>[2x]MHHHHHHAAGIPMNNPAIKRIGNHITKSPEDKREYRGLELANGIKVLLISDPTTDKSSAALDVHIGSLSDPPNIAGLSHFLQHMLFLGTKKYPKENEYSQFLSEHAGSSNAFTSGEHTNYYFDVSHEHLEGALDRFAQFFLSPLFDESAKDREVNAVDSEHEKNVMNDAWRLFQLEKATGNPKHPFSKFGTGNKYTLETRPNQEGIDVRQELLKFHSAYYSSNLMAVVVLGRESLDDLTNLVVKLFSEVENKNVPLPEFPEHPFQEEHLKQLYKIVPIKDIRNLYVTFPIPDLQKYYKSNPGHYLGHLIGHEGPGSLLSELKSKGWVNTLVGGQKEGARGFMFFIINVDLTEEGLLHVEDIILHMFQYIQKLRAEGPQEWVFQELKDLNAVAFRFKDKERPRGYTSKIAGILHYYPLEEVLT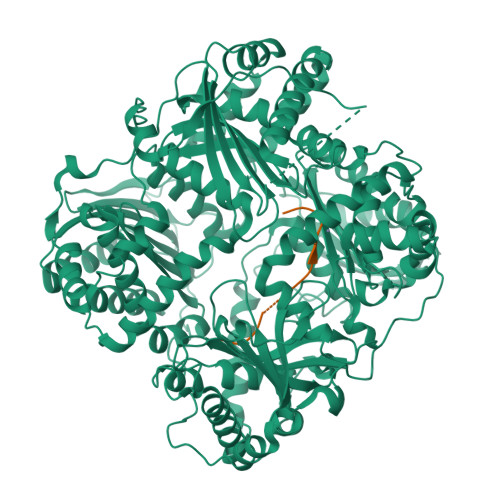AEYLLEEFRPDLIEMVLDKLRPENVRVAIVSKSFEGKTDRTEEWYGTQYKQEAIPDEVIKKWQNADLNGKFKLPTKNEFIPTNFEILPLEKEATPYPALIKDTAMSKLWFKQDDKFFLPKANLNFEFFSPFAYVDPLHSNMAYLYLELLKDSLNEYAYAAELAGLSYDLQNTIYGMYLSVKGYNDKQPILLKKIIEKMATFEIDEKRFEIIKEAYMRSLNNFRAEQPHQHAMYYLRLLMTEVAWTKDELKEALDDVTLPRLKAFIPQLLSRLHIEALLHGNITKQAALGIMQMVEDTLIEHAHTKPLLPSQLVRYREVQLPDRGWFVYQQRNEVHNNSGIEIYYQTDMQSTSENMFLELFAQIISEPAFNTLRTKEQLGYIVFSGPRRANGIQGLRFIIQSEKPPHYLESRVEAFLITMEKSIEDMTEEAFQKHIQALAIRRLDKPKKLSAESAKYWGEIISQQYNFDRDNTEVAYLKTLTKEDIIKFYKEMLAVDAPRRHKVSVHVLAREMDSNPVVGEFPAQNDINLSQAPALPQPEVIQNMTEFKRGLPLFPLVKPHINFMAAKL;>APMGSDPPTACCFSYTARKLPRNFVVDYYETSSLCSQPAVVFQTKRSKQVCADPSESWVQEYVYDLELN[2x]> MIAQGQTLPNATLSQLTKEGMVHHPVLELFAGKKVVLFAVPGAFTPTDSEAHLPGYIVLADQLKAKGVDLIASVSVNDAFVMKAWGEAQNAEEILMLADGDASFTKALGLEMDTAGFGGLRSQRY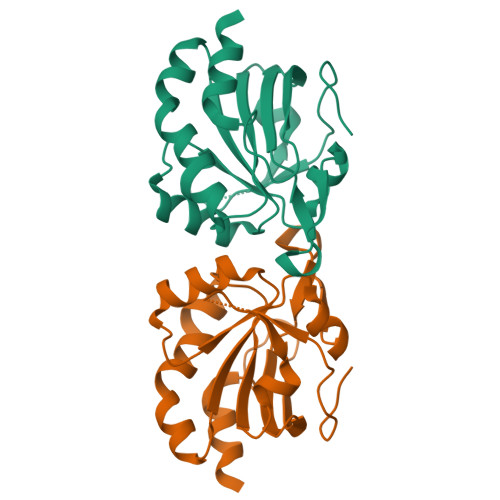AMIIDNGVVTTLNVEAPKSFEVSNAETILAALEHHHHHH>GSHMETVFTEKAPKPVGPYS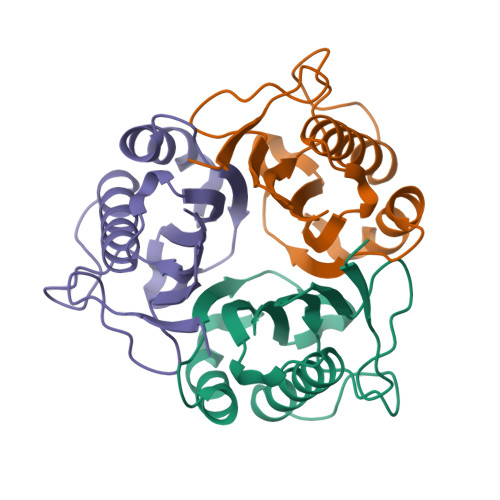QAIKVGNTLYVSGQIPIDPRTNEIVKGDIKVQTRQVLDNIKEIVKAAGFSLSDVAMAFVFLKDMNMFNDFNSVYAEYFKDKPPARVTVEVSRLPKDALIEIAVICSKG[2x]> MFKRLMMVALLVIAPLSAATAADQTNPYKLMDEAAQKTFDRLKNEQPQIRANPDYLRTIVDQELLPYVQVKYAGALVLGQYYKSATPAQREAYFAAFREYLKQAYGQALAMYHGQTYQIAPEQPLGDKTIVPIRVTIIDPNGRPPVRLDFQWRKNSQTGNWQAYDMIA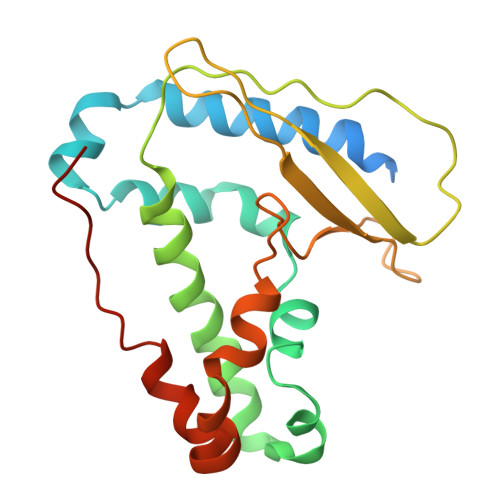EGVSMITTKQNEWGTLLRTKGIDGLTAQLKSISQQKITLEEKK>[3x]MAVPETRPNHTIYINNLNEKIKKDELKKSLHAIFSRF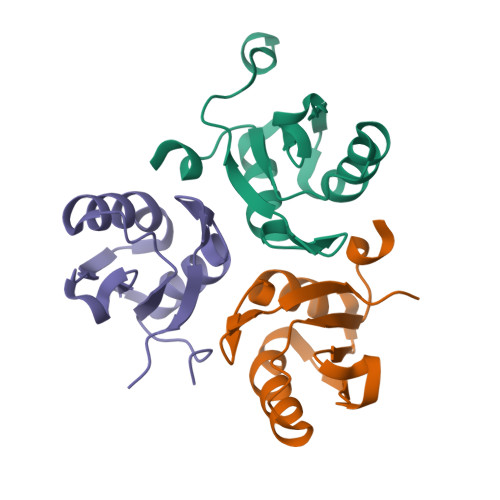GQILDILVSRSLKMRGQAWVIFKEVSSATNALRSMQGFPFYDKPMRIQYAKTDSDIIAKMK1-benzyl-2-phenyl-1H-benzimidazole | C20 H16 N2 | 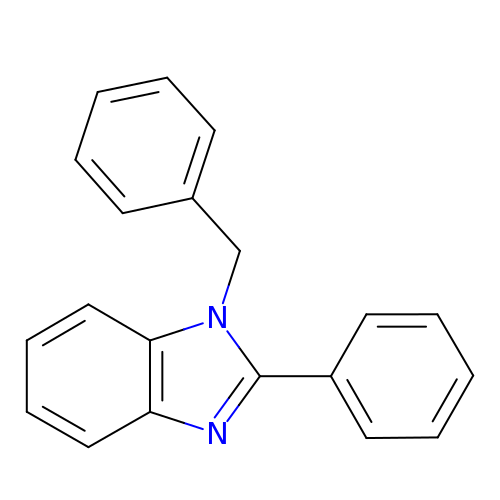LCFXRSKBJWQHON-UHFFFAOYSA-N> ADTYAATRYPVILVHGLAG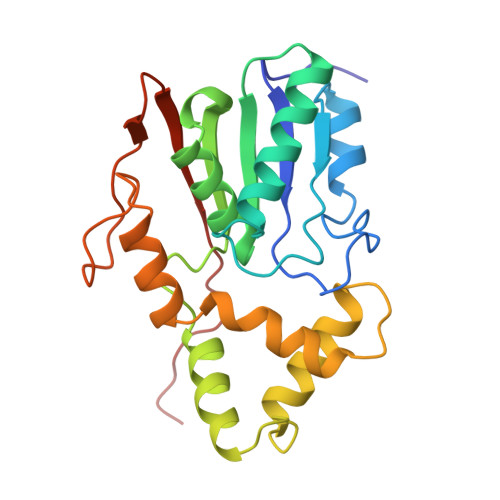TDKFANVVDYWYGIQSDLQSHGAKVYVANLSGFQSDDGPNGRGEQLLAYVKQVLAATGATKVNLIGHSQGGLTSRYVAAVAPQLVASVTTIGTPHRGSEFADFVQDVLKTDPTGLSSTVIAAFVNVFGTLVSSSHNTDQDALAALRTLTTAQTATYNRNFPSAGLGAPGSCQTGAATETVGGSQHLLYSWGGTAIQPTSTVLG>MIRSVVIVGGGTAGWMTASYLKAAFDDRIDVTLVESGNVRRIGVGEATFSTVRHFFDYLGLDEREWLPRCAGGYKLGIRFENWSEPGEYFYHPFERLRVVDGFNMAEWWLAVGDRRTSFSEACYLTHRLCEAKRAPRMLDGSLFASQVDESLGRSTLAEQRAQFPYAYHFDADEVARYLSEYAIARGVRHVVDDVQHVGQDERGWISGVHTKQHGEISGDLFVDCTGFRGLLINQTLGGRFQSFSDVLPNNRAVALRVPRENDEDMRPYTTATAMSAGWMWTIPLFKRDGNGYVYSDEFISPEEAERELRSTVAPGRDDLEANHIQMRIGRNERTWINNCVAVGLSAAFVEPLESTGIFFI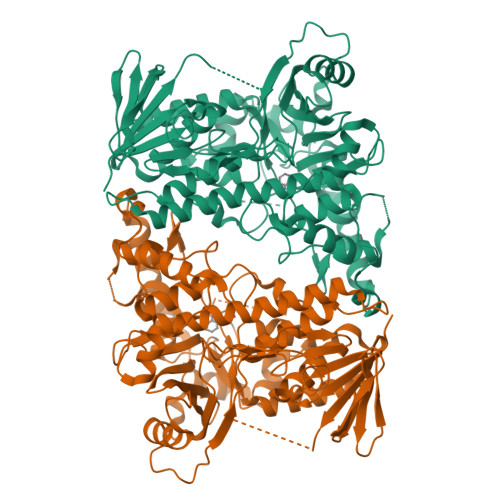QHAIEQLVKHFPGERWDPVLISAYNERMAHMVDGVKEFLVLHYKGAQREDTPYWKAAKTRAMPDGLARKLELSASHLLDEQTIYPYYHGFETYSWITMNLGLGIVPERPRPALLHMDPAPALAEFERLRREGDELIAALPSCYEYLASIQ[4x]> NDDKLYRADSRPPDEIKQSGGLM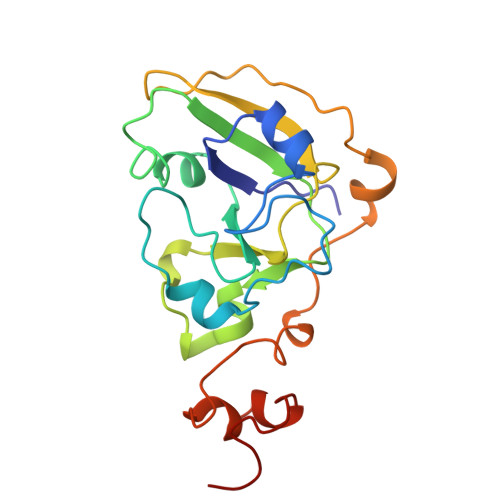PRGQSEYFDRGTQMNINLYDHARGTQTGFVRHDDGYVSTSISLRSAHLVGQTILSGHSTYYLYVLATAPNMFNVNDVLGAYSPHPDEQEVSALGGIPYSQIYGWYRVHFGVLDEQLHRNRGYRDRYYSNLDIAPAADGYGLAGFPPEHRAWREEPWIHHAPPGCGNAPRSS Cilia and flagella-associated protein 410 (CFAP410) localizes at the basal body of cilia/flagella and plays essential roles in ciliogenesis, neuronal development and DNA damage repair. CFAP410 is a bimodular protein comprising two folded domains, i.e. NTD and CTD, which are connected through a variable unstructured loop. All these three crystal structures show a similar homotetrameric arrangement, with each monomer consisting of two α helices that form an open nutcracker-like conformation. Two CTDs first form an intercalated homodimer, and two such dimers further assemble into a tetramer by packing head-to-head through their first helices.

The CTD truncations that finally generated well-diffracting crystals were fragments covering residues 256–295, 212–246 and 213–246 of H. sapiens, T. brucei and C. reinhardtii CFAP410 proteins, respectively. However, those of TbCFAP410 and CrCFAP410 only partially dissolved in the buffer. We, therefore, carried out refolding for the insoluble polypeptides using the following protocol. CrCFAP410-CTD was crystallized in a condition containing 0.02 M CaCl2, 0.1 M sodium acetate (pH 5.0) and 30% (v/v) 2-methyl-2,4-pentanediol at 4°C. Those of HsCFAP410-CTD and CrCFAP410-CTD were determined subsequently by molecular replacement using the crystal structure of TbCFAP410-CTD as a search template. To find out whether and how these highly conserved Leu and Ala residues contribute to the formation of the tetramer, we first examined the wild-type and mutants A219E and L224P of CrCFAP410-CTD using the static light scattering (SLS) method. Our data demonstrated that the wild-type protein formed a tetramer as revealed in the crystal structure, but mutant A219E became a dimer. Surprisingly, mutant L224P completely disrupted the oligomeric structure and formed only a monomer.

>[4x]STKNILYAVMALLGELEDEDLVYVRREIEQRIGGR> SNAGGGGMTRVTVQTAGVHYKWQMPDQLTQQLRLAHDLREDLVTLEYEYEDAVKAVWSSYPAVAALEAQVAELDERASELASTVKEEKSRQRTKRPSHPAVAQLAETRAQLKAAKASRREAIASVRDEATERLRTISDERYAAQKQLYRDYCTDGLLYWATFNAVLDHHKTAVKRIAAHRKQGRAAQLRHHRWDGTGTISVQLQRQATDPARTPAIIADADTGKWRSSLIVPWVNPDVWDTMDRASRRKAGRVVIRMRCGSSRNPDGTKTSEWIDVPVQQHRMLPADADITAAQLTVRREGADLRATIGITAKIPDQGEVDEGPTIAVHLGWRSSDHGTVVATWRSTEPLDIPETLRGVITTQSAERTVGSIVVPHRIEQRVHHHATVASHRDLAVDSIRDTLVAWLTEHGPQPHPYDGDPITAASVQRWKAPRRFAWLALQWRDTPPPEGADIAETLEAWRRADKKLWLESEHGRGRALRHRTDLHRQVAAYFAGVAGRIVVDDSDIAQIAGTAKHSELLTDVDRQIARRRAIAAPGMLRAAIVAA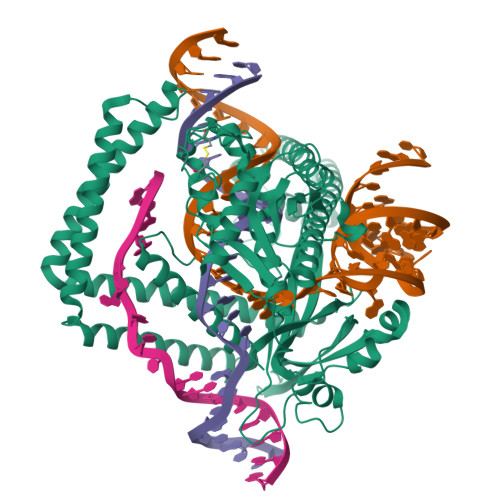ATRDEVPTTTVSHTGLSRVHAACGHENPADDRYLMQPVLCDGCGRTYDTDLSATILMLQRASAATSN> XXTWEA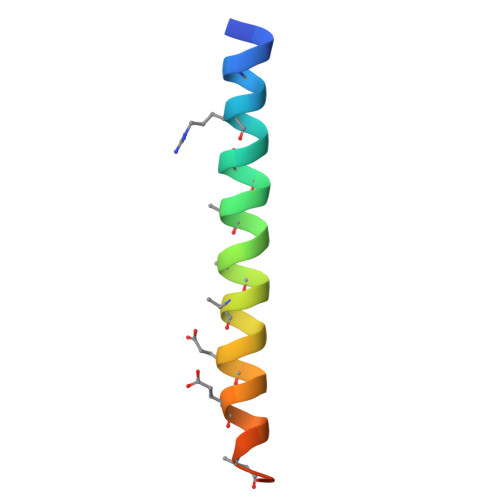WDRAIAEYAARIEALIRAAQEQQEKNEAALRELX>QGTGCSVEIINSNQVSVGS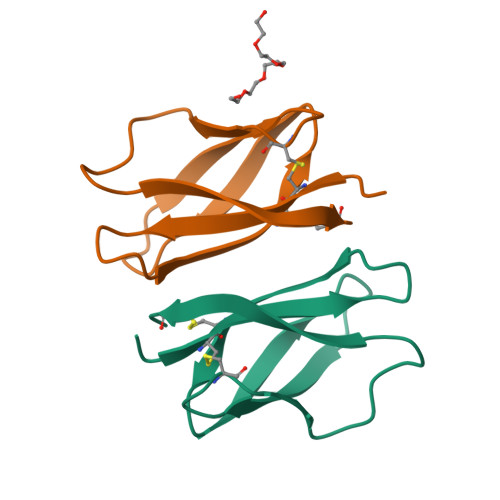GCARINSVTNIGDNQGRRWGVLANSSCGLSTTQNLPSGWSLRQTGFCNA[2x]> GPHMRTFFVGGNWKANPKTVQEAEKLVEMLNGAKVEGNVEVVVAAPFAFLPTLQQKLRKDWKVSAENVFTKPNGAFTGEVTVPMIKSFGIEWTILGHSERRDILKEDDEFLAAKAKFALENGMKIIYCCGEHLSEREAGKASEFVSAQIEKMIPAIPAGKWDDVVIAYEPIWAIGTGKVASTQDAQEMCKVIRDILAAKVGADIANKVRILYGGSVKPNNCNELAA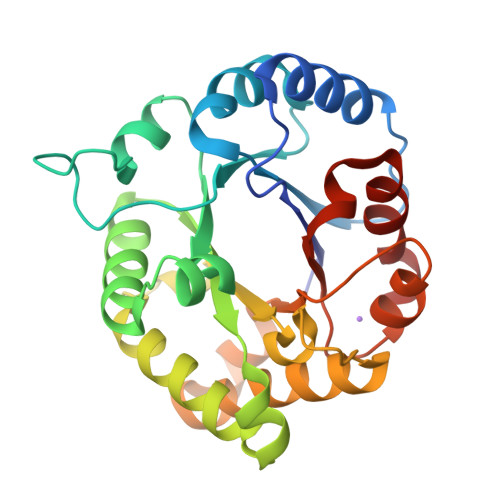CPDVDGFLVGGASLEAGFINIVNSNVHSK> GSHMLELPHEKDKPVAEPIPICSFCLGTKEQNREKKPEELISCADCGNSGHPSCLKFSPELTVRVKALRWQCIECKTCSSCRDQGKNADNMLFCDSCDRGFHMEC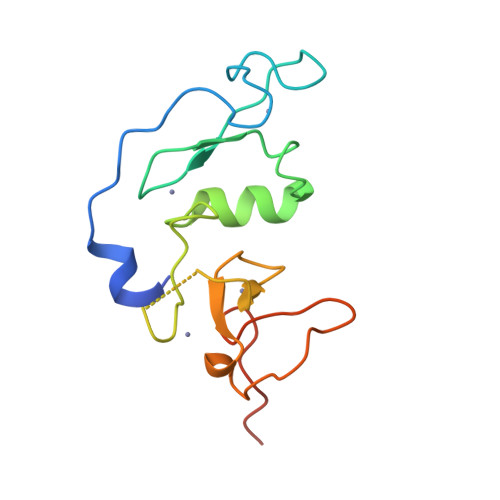CDPPLTRMPKGMWICQICRPRKKGRKLLQKK(2S)-1-(pyrrolidin-1-yl)-3-(9H-thioxanthen-9-yl)propan-2-ol | 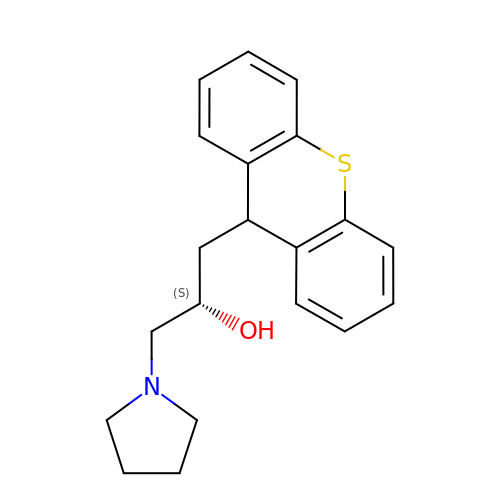C20 H23 N O S | SJCVUEZFZDNDKT-HNNXBMFYSA-N>[3x]SS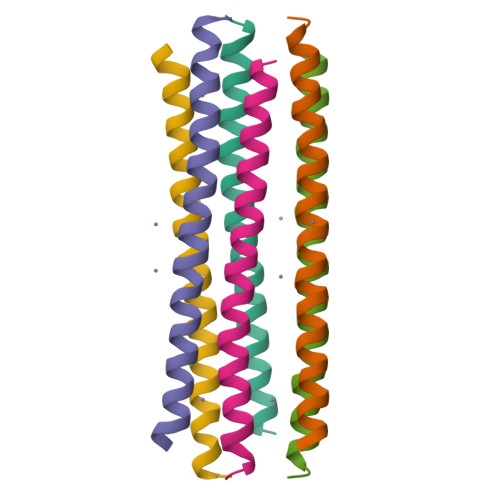LLEKGLDGAKKAVGGLGKLGKDAVEDLESVGKGAVHDVKDVLDSVL> MNDIAHNLAQVRDKISAAATRCGRSPEEITLLAVSKTKPASAIAEAIDAGQRQFGENYVQEGVDKIRHFQELGVTGLEWHFIGPLQSNKSRLVAEHFDWCHTIDRLRIATRLNDQRPAELPPLNVLIQINISDENSKSGIQLAELDELAAAVAELPRLRLRGLMAIPAPESEYVRQFEVARQMAVAFAGLKTRYPHIDTLSLGMSDDMEAAIAAGSTMVRIGTAIFGARDYSKK

The pyridoxal 5′‐phosphate (PLP) homeostasis protein (PLPHP) is a ubiquitous member of the COG0325 family with apparently no catalytic activity. Although the actual cellular role of this protein is unknown, it has been observed that mutations of the PLPHP encoding gene affect the activity of PLP‐dependent enzymes, B6 vitamers and amino acid levels. Here we report a detailed characterization of the Escherichia coli ortholog of PLPHP (YggS) with respect to its PLP binding and transfer properties, stability, and structure. YggS binds PLP very tightly and is able to slowly transfer it to a model PLP‐dependent enzyme, serine hydroxymethyltransferase.

PLP binding to YggS elicits a conformational/flexibility change in the protein structure that is detectable in solution but not in crystals.>MKQNINIGNVVDDGTGDYLRKGGIKINENFDELYYELGDGDVPYSAGAWKTYNASSGQTLTAEWGKSYAINTSSGRVTINLPKGTVNDYNKVIRARDVFATWNVNPVTLVAASGDTIKGSAVPVEINVRFSDLELVYCAPGRWEYVKNKQIDKITSSDISNVARKEFLVEVQGQTDFLDVFRGTSYNVNNIRVKHRGNELYYGDVFSENSDFGSPGENEGELVPLDGFNIRLRQPCNIGDTVQIETFMDGVSQWRSSYTRRQIRLLDSKLTSKTSLEGSIYVTDLSTMKSIPFSAFGLIPGEPINPNSLEVRFNGILQELAGTVGMPLFHCVGADSDDEVECSVLGGTWEQSHTDYSVETDENGIP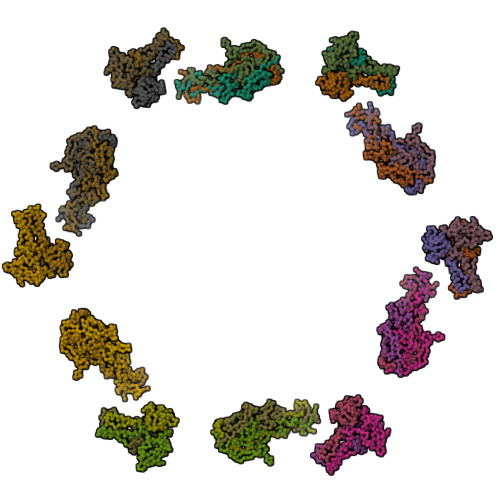EILHFDSVFEHGDIINITWFNNDLGTLLTKDEIIDETDNLYVSQGPGVDISGDVNLTDFDKIGWPNVEAVQSYQREFNAVSNIFDTIYPIGTIYENAVNPNNPVTYMGFGSWKLFGQGKVLVGWNEDISDPNFALNNNDLDSGGNPSHTAGGTGGSTSVTLENTNLPATETDEEVLIVDENGSVIVGGCQYDPDESGPIYTKYREAKASTNSTHTPPTSITNIQPYITVYRWIRIA[18x]>[2x]MSNKLFPPQIKVAATYMRGGTSKGVFFRLQDLPEAAQVPGPARDALLLRVIGSPDPYAKQIDGMGGATSSTSKTVILSHSSKANHDVDYLFGQVSIDKPFVDWSGNCGNLTAAVGAFAISNGLIDAARIPRNGVCTVRIWQANIGKTIIAHVPITDGAVQETGDFELDGVTFPAAEVQIEFMNPAADDDGEGGCMFPTGNLVDVLE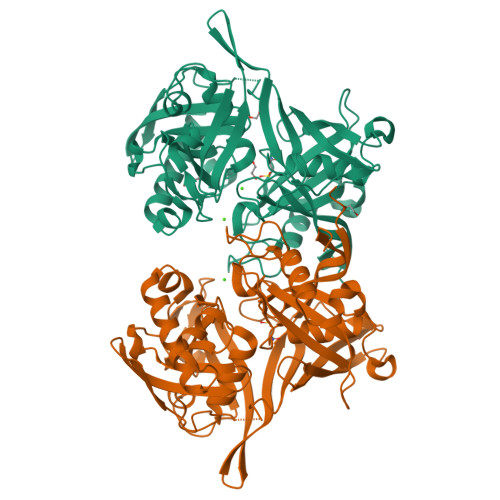VPGIGRFNATMINAGIPTIFINAEDLGYTGTELQDDINSDNAALAKFETIRAHGALRMGLIKHIDEAASRQHTPKIAFVAPPKSYASSSGKTVAAEDVDLLVRALSMGKLHHAMMGTAAVAIGTAAAIPGTLVNLAAGGGEKEAVRFGHPSGTLRVGAQAVQENGEWTVIKAIMSRSARVLMEGFVRVPKP2-(piperazin-1-yl)-4-(trifluoromethyl)pyrimidine | C9 H11 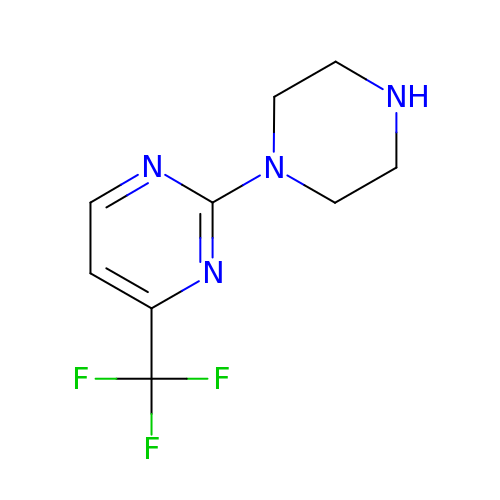F3 N4 | WBJVPAABGFBMJQ-UHFFFAOYSA-N> LPQDRGFLVVQGD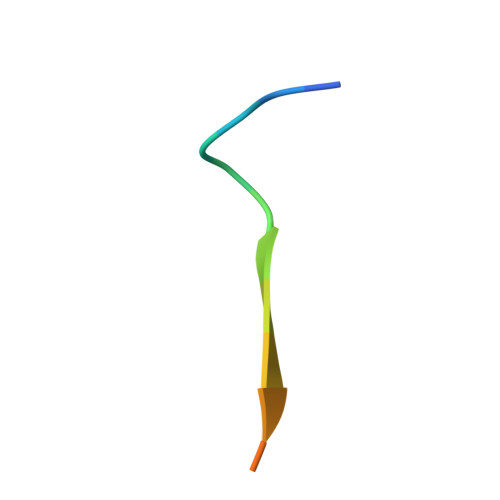PR> MSNRFFQKFYLRCGNCSAIQRSAQGYQPIANPILFKSDEHCRNYHDEQRRAAGYSGMVVTCRCHRCERVHSNWKVLDAQQFLDAKLRMTPEERAQR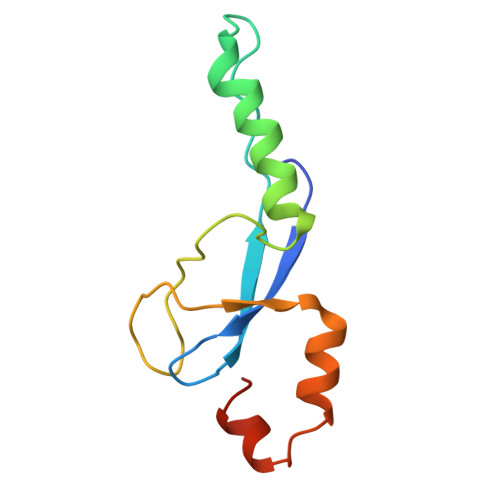LWVSKS The Lon protease is a AAA+ protein found in prokaryotes, archaea, and eukaryotic organelles. Lon is involved in cellular protein homeostasis by degrading damaged or misfolded abnormal proteins, which prevents these unwanted protein species from forming toxic aggregates. Lon is known to form a homohexamer; each protomer is composed of multiple domains, including an N-terminal substrate-binding globular domain (NGD), a long-helix domain (LH), a three-helix bundle (3H), a AAA+ ATPase module, and a protease domain. We show here, using cryo-electron microscopy (cryo-EM), that the activation process of the Lon AAA+ protease may involve a pentameric assembly and a substrate-dependent incorporation of the sixth protomer to form the substrate-pore-loop contacts seen in the translocating state.

To test this hypothesis, we performed single-particle cryo-EM reconstruction of the proteolytically deficient mutant MtaLon-S678A incubated with ADP and the model substrate α-casein. Indeed, 3D reconstruction of the data revealed a substrate-bound hexameric form, which adopts a close-ring structure with the substrate-pore-loop contacts in a right-handed spiral-staircase-like arrangement. Previously, similar close-ring hexameric structures of Lon were only reported with the presence of substrate and ATP analogs. Here, our structural analysis shows that in the substrate-bound state, the sixth protomer Ac6* binds to the pentameric assembly and bridges Ob1 and Ob5 together to form a close-ring hexamer, in which the four substrate-engaged protomers are Ac4-Ob5-Ac6*-Ob1. In this structure, Ac4, Ob5, and Ac6* engage the substrate polypeptide by the pore-loop I (Tyr397) and II (Trp431) residues, but the lowermost Ob1 contacts the substrate by pore-loop I only. The three protomers Ac4, Ob5, and Ac6* are tightly packed. By contrast, the protomers Ob1, Ac2, and Ob3 are only loosely contacted by their AAA+ domains; and their pore loops II are disordered. All of the substrate-binding loops in the proteolytic active sites adopt an active conformation, albeit not as ordered as in the inhibitor- or substrate-bound states with ATPγS. In the close-ring hexameric state, the pore-loop-I Y397 residues of these protomers and Ac6* mediate substrate contacts; together they are aligned on the trajectory. However, when the substrate is present, binding of the substrate to the exposed pore loops of pentamer may induce binding of pore loops of the sixth protomer to the engaged substrate polypeptide presented by pentamer and promote rapid formation of the closed-ring hexamer with stabilized substrate interaction.

>[6x]MRLELPVIPLRNTVILPHTTTPVDVGRAKSKRAVEEAMGADRLIFLVAQRDPEVDDPAPDDLYTWGVQAVVKQAMRLPDGTLQVMVEARARAQVTDYIPGPYLRARGEVFSEIFPIDEAVVRVLVEELKEAFEKYVANHKSLRLDRYQLEAVKGTSDPAMLADTIAYHATWTVAEKQEILELTDLEARLKKVLGLLSRDLERFELDKRVAQRVKEQMDTNQREYYLREQMKAIQKELGGEDGLSDLEALRKKIEEVGMPEAVKTKALKELDRLERMQQGSPEATVARTYLDWLTEVPWSKADPEVLDINHTRQVLDEDHYGLKDVKERILEYLAVRQLTQGLDVRNKAPILVLVGPPGVGKTSLGRSIARSMNRKFHRISLGGVRDEAEIRGHRRTYIGAMPGKLIHAMKQVGVINPVILLDEIDKMSSDWRGDPASAMLEVLDPEQNNTFTDHYLDVPYDLSKVFFITTANTLQTIPRPLLDRMEVIEIPGYTNMEKQAIARQYLWPKQVRESGMEGRIEVTDAAILRVISEYTREAGVRGLERELGKIARKGAKFWLEGAWEGLRTIDASDIPTYLGIPRYRPDKAETEPQVGTAQGLAWTPVGGTLLTIEVAAVPGSGKLSLTGQLGEVMKESAQAALTYLRAHTQDYGLPEDFYNKVDLHVHVPDGATPKDGPAAGITMATAIASALSRRPARMDIAMTGEVSLRGKVMPIGGVKEKLLAAHQAGIHKIVLPKDNEAQLEELPKEVLEGLEIKLVEDVGEVLEYLLLPEPTMPPVVQPSDNRQQPGAGA>[2x]MKSNEHDDCQVTNPSTGHLFDLSSLSGRAGFTAAYSEKGLVYMSICGENENCPPGVGACFGQTRISVGKANKRLRYVDQVLQLVYKDGSPCPSKSGLSYKSVISFVCRPEAGPTNRPMLISLDKQTCTLFFSWHTPLACEQATECSVRNGSSIVDLSPLIHRTGGYEAYDESEDDASDTNPDFYINICQPLNPMHAVPCPAGAAVCKVPIDGPPIDIGRVAGPPILNPIANEIYLNFESSTPCLADKHFNYTSLIAFHCKRGVSMGTPKLLRTSECDFVFEWETPVVCPDEVRMDG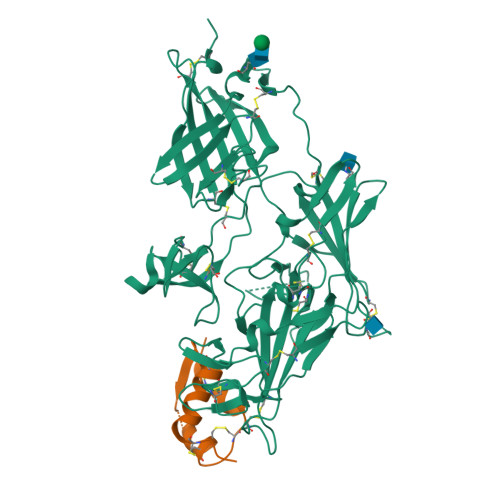CTLTDEQLLYSFNLSSLSTSTFKVTRDSRTYSVGVCTFAVGPEQGGCKDGGVCLLSGTKGASFGRLQSMKLDYRHQDEAVVLSYVNGDRCPPETDDGVPCVFPFIFNGKSYEECIIESRAKLWCSTTADYDRDHEWGFCRHSNSYRTSSIIFKCDEDEDIGRPQVFSEVRGCDVTFEWKTKVVCPPKKLKHHHHHH;>AYRPSETLCGGELVDTLQFVCGDRGFYFSRPASRVSRRSRGIVEECCFRSCDLALLETYCATPAKSE[2x]>SMSSHDGLMVFTGNANPALAQEVVKILGIPLGKAMVSRFSDGEIQVEIQENVRGKDVFVLQSTCAPTNDNLMELMIMVDALKRASAGRITAAIPYFGYARQDRRPRSARVAISAKVVANMLEIAGVERIITMDLHADQIQG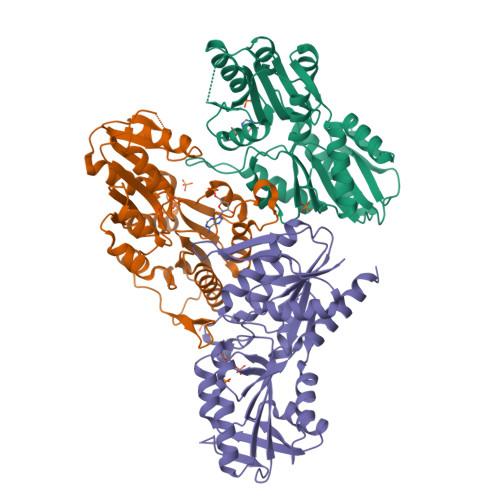FFDIPVDNIYATPILLGDLRKQNYPDLLVVSPDVGGVVRARALAKQLNCDLAIIDKRRPKANVAEVMNIIGEVEGRTCVIMDDMVDTAGTLCKAAQVLKERGAKQVFAYATHPVLSGGAADRIAASALDELVVTDTIPLSAESLACPKIRALSSAGLLAETFSRIRRGDSVMSLFAES[3x]> GAGAGAGAGAGMGQPTTTSLFMRDVMFHRMTGTSQAVNDVATLSGERREIIRRALNKKILVPNILELMPAWPSEFQPNIDEVNVEIDEWLKTVNVAKEKKLKHRARGNYTLLAGIYYPHCRKEKMLALSQFLYWIFFWDDEIDTGGELTEDREGTILCCAETNKCINDCLGPEPNYTPPPGSRGTVEMLYPILRDLRAGLSPVSTMRLKQELHDYVNGVKNQQKVRQEDHLPNPWDHFQMRVDDVGVIPSITQNEYAMDFTLPDWIRRHEAMEEIVLQCTKLTILLNEILSLQKEFRVSQLENLCLLFMNT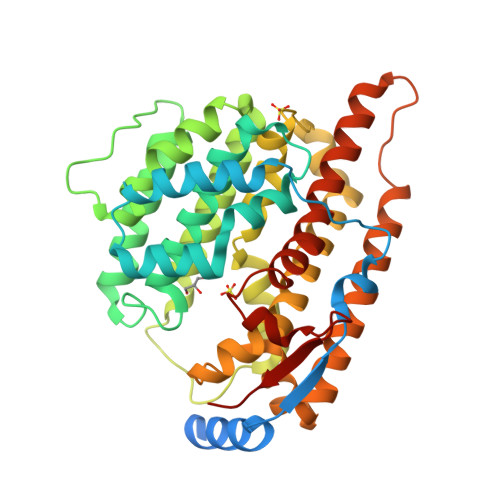YDMSIEQSIHKVLGLLKDHYKICIEAEARLPWSTTDEKLNNNIREYIRGCQRLATGTACWSYNCERYFKLSQLNDQQELLLDLSRT>[3x]MKAVVPTGKIYLGSPFYSDAQRERAAKAKELLAKNPSIAHVFFPFDDGFTDPDEKNPEIGGIRSMVWR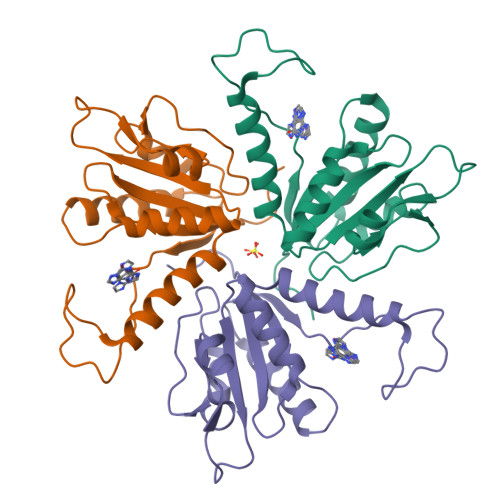DATYQNDLTGISNATCGVFLYDMDQLDDGSAFEIGFMRAMHKPVILVPFTEHPEKEKKMNLMIAQGVTTIIDGNTEFEKLADYNFNECPSNPVRGYGIY6-ethyl-5-{3-[3-methoxy-5-(pyridin-4-yl)phenyl]prop-1-yn-1-yl}pyrimidine-2,4-diamine 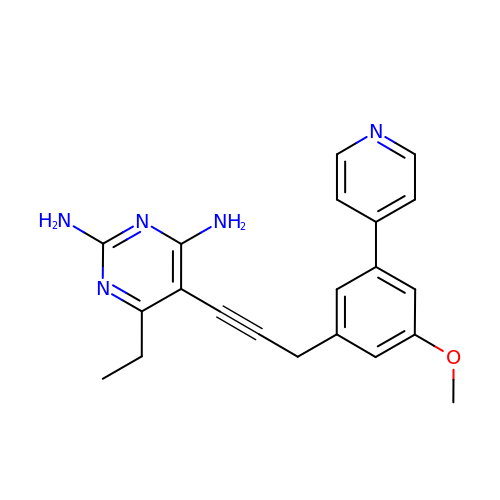| C21 H21 N5 O | COHGVYNMDPBQFR-UHFFFAOYSA-N>MTKTEKKGNIEIEALKDVVVNIGGIEEEEEEWEPMGPTPMPGIVDLRDWDYKLMDRYKPFYAPYCEMCCFCTFGKCDLTGGKKGACGLDMTAQQARFVTIACLIGCSAHTAHGRHMLNEILHIYGDREIDMGTGINIEAPLTRLITGIKPKRLSDFIPVLDYIEEQIAQVMDSVHTGQEGSNIDYESKAFHVGMLDSLGKEVADIVQIVAFDLPKGDPDAPLVEIGMGCIDETKPMLLVIGHNVVPSVSVIDYMREHDLEDKIEVAGICCTAIDTTRYSDRAKIVGSIGRQLRFVRSGIADVIMVDEQCIRADILEQAKRTHAPLIATNDKALYGLVDRTDDSADDIITILVSGKEPGVVILDPVKAGEVAVRLVQIMHEKRKGLVHLPTDEEFKEYVEMCQNCDANCVIACPQGLPIGEANKAAAAGNIEPLAELFDLCVGCGRCEQVCKKHIPIVDVIHKAALPLVRAEKGMIRVGRGPVLDTEIRNVGAPLVLGTIPGIIAIVGCGNYPNGTKDVYIMAKEFVERKYIVVLTGCGAMDAALYRDEDGKTLYEKYPGDFDGGCIVNIGSCVSNAHIHDAAIKVASIFARRNIRANYAEIADYILNRVGACGMAWGAMSQKAASIASGVNRIGIPVVIGPHGWKYRRAYLGRKDVDRDWMVYDARDGSKVRIEPAPEHLLVAADTLEEAIPLMARLCFRPTDNSMGRQVKLTHYMDLSMKYLGKYPDDWPVFVRTEADLPLAKKEEYLRILKEDYGWDVDLEAKKIISGPIRKFDVSFDATNLEQLIRENK[2x];>MKFDEKGSIIDLETKVVYSNICCYCGACGAFCTEYISYENGTPVTKQKCFEIHGACFDFCPRTFLPVLEMERELFGEVRSDWELGYYTDIVTARATNPEILEKGQNGGVVTALLTHLIDEGKIDAACITGRSDDEPWKPEPLVATTRDEILKGAGSNYEQCPAIMGVGEALANGSENIAMVGLPCHIQAMRKIQLSKAFDVGASRVKYAIGLLCTETFDRDLLHAKLREMKIKAEDVKKFDIGEGKFKVFTEEGVRTEKIATMKSCMRDGCKVCYDFAAELADISVGSIGSEEGWNTVLIRSKAGKELIDEAEKAKVIEVKPLNEASIQSVKDLASRKKSENMDNIVEIAGATKILHLAVKPQELSLLLG[2x];>MNIPFDIGNISGPEMGRIATPEALGRAIKNAKRPLLVVGSEILEDGLIDRAIAIGKKGIPIAATAHSIKGFVDAGYTDNVYMVGLHELANNIKSPDWMGFDGKGGYDLVAVLGGIYYSTSQFLISIKNCATDPLVRAISIDRYYHIAARMTFDNISRKRTDEFKEMLDRVVQSI[2x]

Here, we study the molecular basis of the CO2-generating steps of anaerobic ethane oxidation by characterising native enzymes of the thermophile Candidatus Ethanoperedens thermophilum obtained from microbial enrichment. We perform biochemical assays and solve crystal structures of the CO dehydrogenase and formylmethanofuran dehydrogenase complexes, showing that both enzymes deliver electrons to the F420 cofactor. Both multi-metalloenzyme harbour electronic bridges connecting CO and formylmethanofuran oxidation centres to a bound flavin-dependent F420 reductase. Based on the crystal structures, enzymatic activities, and metagenome mining, we propose a model in which the catabolic oxidising steps would wire electron delivery to F420 in this organism.

The structure of the CODH component of the ACDS was obtained by X-ray crystallography and refined to a 1.89-Å resolution. The α2ε2 core of the CODH component can be reliably superposed on the homologous structure from Methanosarcina barkeri, also obtained from dissociation from the ACDS complex. While the α subunit exhibits high structural conservation with the homologue from M. barkeri, the ε subunit slightly differs due to local reorganisations to accommodate the ζ subunit. Each α/ε interface of the complex from Ca. E. thermophilum accommodates an ion in close proximity to the [4Fe-4S] cluster 3 (modelled as a K atom). In the structure of M. barkeri, the respective position is empty, suggesting that the additional ion may be a thermophilic adaptation of the enzyme to optimise the stability between the subunits. The C-cluster operating the CO-oxidation was obtained in a non-carbonylated state with the CO site vacant in both α subunits occupying the asymmetric unit. The ζ subunit is positioned at the intersection of α and ε subunits. It is composed of a ferredoxin domain in its N-terminal part (1–83, containing two [4Fe-4S] clusters), an F420-reductase domain (84–349, containing one [4Fe-4S] cluster and the flavin adenine dinucleotide, FAD), and a C-terminal extension promoting the homodimeric interface (350–370). The anchoring of the ζ subunit to the α2ε2 core through its N-terminal domain offers a structural template to picture how the electrons from the distal cluster of the α subunit (cluster 4) will be transferred on the distal cluster of the ζ subunit (cluster 5).2,2-dimethyl-N-(2,4,6-trimethoxyphenyl)dodecanamide | C23 H39 N O4 | 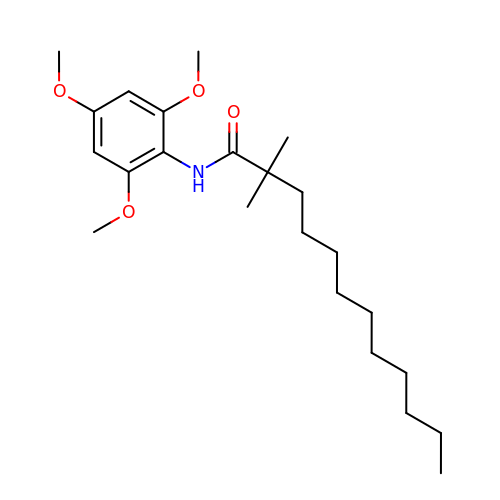WAFNZAURAWBNDZ-UHFFFAOYSA-N> GAFLDKPKMEKHNAQGQGNGLRYGLSSMQGWRVEMEKAHTAVIGLPSGLESWSFFAVYDGHAGSQVAKYCCEHLLDHITNNQDFKGSAGAPSVENVKNGIRTGFLEIDEHMRVMSEKKHGADRSGSTAVGVLISPQHTYFINCGDSRGLLCRNRKVHFFTQDHKPSNPLEKERIQNAGGSVMIQRVNGSLAVSRALGDFDYKCVHGKGPTEQLVSPEPEVHDIERSEEDDQFIILACDGIWDVMGNEELCDFVRSRLEVT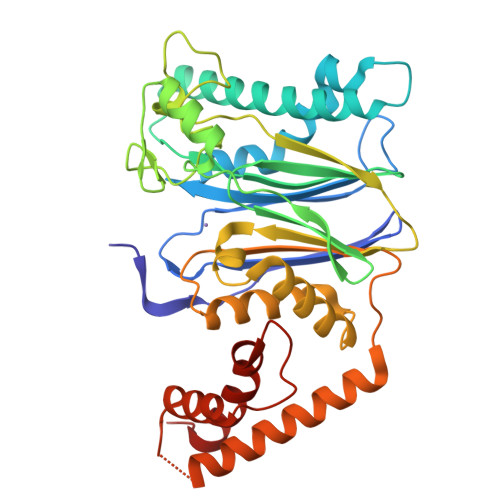DDLEKVCNEVVDTCLYKGSRDNMSVILICFPNAPKVSPEAVKKEAELDKYLECRVEEIIKKQGEGVPDLVHVMRTLASENIPSLPPGGELASKRNVIEAVYNRLNPY Heme oxygenase (HO) converts heme to carbon monoxide, biliverdin, and free iron, products that are essential in cellular redox signaling and iron recycling. In higher plants, HO is also involved in the biosynthesis of photoreceptor pigment precursors. Although the enzymatic reactions carried out by bacterial, mammalian, and photosynthetic HOs are the same, there is a difference in the electron donor required for the reactions, that is, ferredoxin (Fd) is used by photosynthetic HOs, whereas NADPH–cytochrome P450 reductase (CPR) is used by mammalian HOs. Despite many common enzymatic reactions, the amino acid sequence identity between plant-type and other HOs is exceptionally low (∼19.5%), and amino acids that are catalytically important in mammalian HO are not conserved in plant-type HOs.

In this study, we have determined the high-resolution crystal structure of GmHO-1 complexed with heme at a resolution of 1.06 Å, which is the highest resolution for an HO structure reported to date. We therefore adopted the iron single-wavelength anomalous dispersion (Fe-SAD) method for phase determination and successfully solved the structure with refinement finally up to a resolution of 1.06 Å using SHELXL and COOT. The GmHO-1 structure comprises four 310 helices (residues 45–47, 50–52, 84–89, and 172–174) and eight α-helices designated as α1 (20–29), α2 (57–80), α3 (96–110), α4 (119–134), α5-1 (136–151), α5-2 (153–166), α6 (180–196), and α7 (200–224). The heme molecule bound to GmHO-1 is sandwiched between proximal (α1) and distal (α5) helices with axial ligation from His30 residue, consistent with previous data from electron paramagnetic resonance measurements. New features of the GmHO-1 structure include the shorter α1 helix and an additional irregularly structured region continuing from α1, which has not been observed in any other HO structures. To accommodate this novel irregularly structured region near the heme-binding site, the α7 helix (corresponding to α9 in HmuO or α8 in hHO-1) has become a curvilinear helix. Because the C-terminal α7 helix is curved and becomes a curvilinear helix, the last half of this helix forms an unexpected tunnel, together with the novel irregularly structured region. Although the plant-type HO lacks the conserved Asp and Arg residues for the hydrogen-bonding network observed in hHO-1 and HmuO, it has an alternative hydrogen-bonding network formed by Ala149 and His150. On the proximal side, the imidazole ring of the ligating His30 residue, which is rotated approximately 160°, and the δ-nitrogen form a new hydrogen bond to the carbonyl oxygen of Ala26, whereas the δ-nitrogen of the other HOs forms a hydrogen bond with the side chain of a Glu residue (Glu24 in HmuO and Glu29 in rHO-1 and hHO-1), supporting the plant-type–specific accommodation of heme near the N terminus. Interestingly, the back and side walls of the heme pocket are negatively charged in GmHO-1, whereas the other HOs have positively charged walls.

> MSAATAETPKKKGESKGFVEEMRFVAMRLHTRDQAREGEKEVKQPEEKAVTKWDPSVEGYLKFLVDSKLVYDTLEKIVQEAPHPSYAEFRNTGLERSASLAEDLEWFKEQGYTIPEPSSPGLTYAQYLKELSVKDPQAFICHFYNIYFAHSAGGRMIGKKVAEKLLNNKALEFYKWDDDLPRLLQNVRDKLNKVAEPWSREEKDHCLEETEKSFKLSGEILRLILS>GQNVPEGVIGAFKEGNSQELNKYLGDKVDLIIQNKSTHADKRTAEGTMAAFFSNHKVGSFNVNHQGKRDESGFVIGILMTANGNFRVNCFFRKVQNKYVIHQI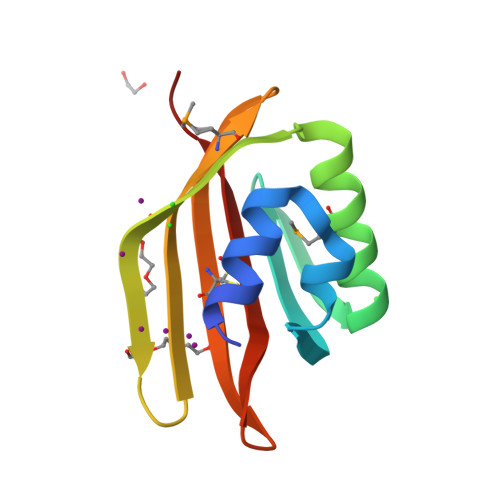RIDKTDE[2x]> ADPPVVNTAYGRVRGVRRELNNEILGPVVQFLGVPYATPPLGARRFQPPEAPASWPGVRQATTLPPACPQNLHGALPAIMLPVWFTDNLEAAATYVQNQSEDCLYLNLYVPTEDGPLTKKRDEA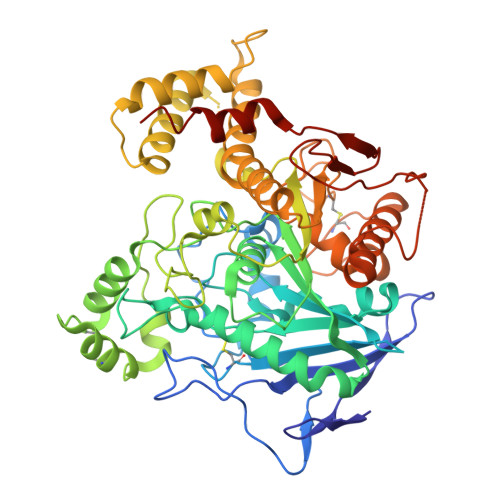TLNPPDTDIRDPGKKPVMLFLHGGSYMEGTGNMFDGSVLAAYGNVIVATLNYRLGVLGFLSTGDQAAKGNYGLLDQIQALRWLSENIAHFGGDPERITIFGSGAGASCVNLLILSHHSEGLFQKAIAQSGTAISSWSVNYQPLKYTRLLAAKVGCDREDSAEAVECLRRKPSRELVDQDVQPARYHIAFGPVVDGDVVPDDPEILMQQGEFLNYDMLIGVNQGEGLKFVEDSAESEDGVSASAFDFTVSNFVDNLYGYPEGKDVLRETIKFMYTDWADRDNGEMRRKTLLALFTDHQWVAPAVATAKLHADYQSPVYFYTFYHHCQAEGRPEWADAAHGDELPYVFGVPMVGATDLFPCNFSKNDVMLSAVVMTYWTNFAKTGDPNQPVPQDTKFIHTKPNRFEEVVWSKFNSKEKQYLHIGLKPRVRDNYRANKVAFWLELVPHLHNLVPR(1S,5S,6R)-10-[(3,5-dichlorophenyl)sulfonyl]-5-[(1S)-1,2-dihydroxyethyl]-3-[2-(3,4-dimethoxyphenoxy)ethyl]-3,10-diazabicyclo[4.3.1]decan-2-one 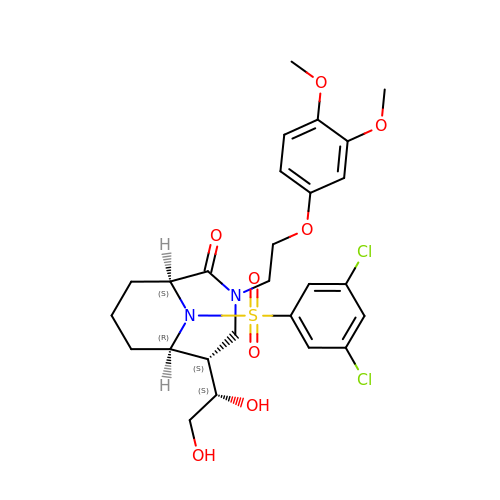| C26 H32 Cl2 N2 O8 S | JKYLGBPUGDRSCP-GSPCLOLRSA-N> GSSGSSGEGELRLGERVLVVGQRLGTIRFFGTTNFAPGYWYGIELEKPHGKNDG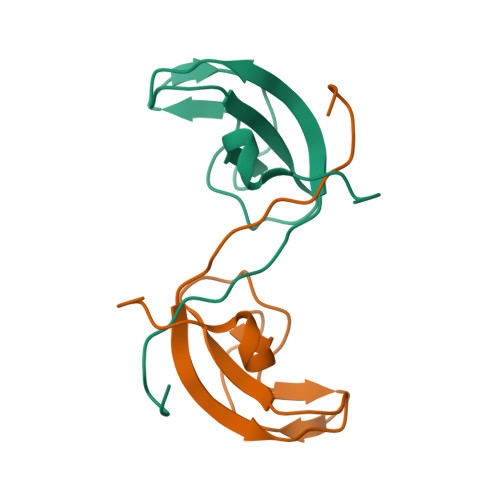SVGGVQYFSCSPRYGIFAPPSRVQRVTDSLDTLSEISGPSSG N-(6-ACETAMIDOHEXYL)ACETAMIDE 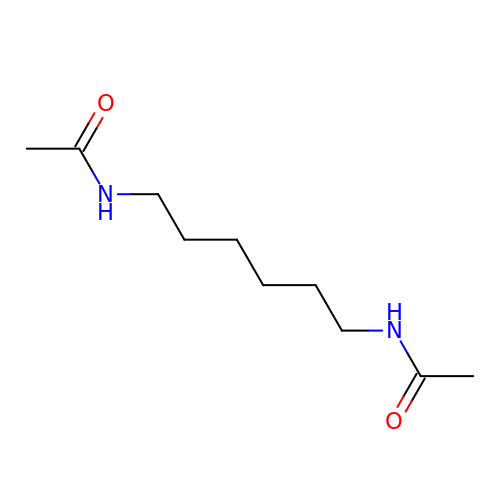| C10 H20 N2 O2 | BNQSTAOJRULKNX-UHFFFAOYSA-N> GAVSIEPRINVGSRFQAEIPLMRDRALAAADPHKADLVWQ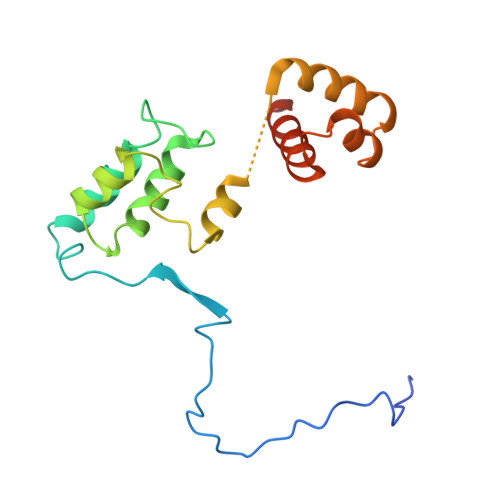PWEDLESSREKQRQVEDLLTAACSSIFPGAGTNQELALHCLHESRGDILETLNKLLLKKPLRPHNHPLATYHYTGSDQWKMAERKLFNKGIAIYKKDFFLVQKLIQTKTVAQCVEFYYTYKKQVKIGRNGTLT>PSAAIYNIDTSSESPDHYLVDHTLDGRVLFPATGYLSIVWKTLARALGLGVEQLPVVFEDVVLHQATILPKTGTVSLEVRLLEASRAFEVSENGNLVVSGKVYQWDDPDPRLFDHPESPTPNPTEPLFLAQAEVYKELRLRGYDYGPHFQGILEASLEGDSGRLLWKDNWVSFMDTMLQMSILGSAKHGLYLPTRVTAIHIDPATHRQKLYTLQDKAQVADVVVSRWLRVTVAGGVHISGLHTESAPRRQQEQQVPILEKFCFTPHTEEGCLSERAALQEELQLCKGLVQALQTKVTQQGLKMVVPGLDGAQIPRDPSQQELPRLLSAACRLQLNGNLQLELAQVLAQERPKLPEDPLLSGLLDSPALKACLDTAVENMPSLKMKVVEVLAGHGHLYSRIPGLLSPHPLLQLSYTATDRHPQALEAAQAELQQHDVAQGQWDPADPAPSALGSADLLVCNCAVAALGDPASALSNMVAALREGGFLLLHTLLRGHPLGDIVAFLTSTEPQYGQGILSQDAWESLFSRVSLRLVGLKKSFYGSTLFLCRRPTPQDSPIFLPVDDTSFRWVESLKGILADEDSSRPVWLKAINCATSGVVGLVNCLRREPGGNRLRCVLLSNLSSTSHVPEVDPGSAELQKVLQGDLVMNVYRDGAWGAFRHFLLEEDKPEEPTAHAFVSTLTRGDLSSIRWVCSSLRHAQPTCPGAQLCTVYYASLNFRDIMLATGKLSPDAIPGKWTSQDSLLGMEFSGRDASGKRVMGLVPAKGLATSVLLSPDFLWDVPSNWTLEEAASVPVVYSTAYYALVVRGRVRPGETLLIHSGSGGVGQAAIAIALSLGCRVFTTVGSAEKRAYLQARFPQLDSTSFANSRDTSFEQHVLWHTGGKGVDLVLNSLAEEKLQASVRCLATHGRFLEIGKFDLSQNHPLGMAIFLKNVTFHGVLLDAFFNESSADWREVWALVQAGIRDGVVRPLKCTVFHGAQVEDAFRYMAQGKHIGKVVVQVLAEEPEAVLKGAKPKLMSAISKTFCPAHKSYIIAGGLGGFGLELAQWLIQRGVQKLVLTSRSGIRTGYQAKQVRRWRRQGVQVQVSTSNISSLEGARGLIAEAAQLGPVGGVFNLAVVLRDGLLENQTPEFFQDVCKPKYSGTLNLDRVTREACPELDYFVVFSSVSCGRGNAGQSNYGFANSAMERICEKRRHEGLPGLAVQWGAIGDVGILVETMSTNDTIVSGTLPQRMASCLEVLDLFLNQPHMVLSSFVLAEKAAAYRDRDSQRDLVEAVAHILGIRDLAAVNLDSSLADLGLDSLMSVEVRQTLERELNLVLSVREVRQLTLRKLQELSSKADEASELACPTPKEDGLAQQQTQLNLRSLLVNPEGPTLMRLNSVQSSERPLFLVHPIEGSTTVFHSLASRLSIPTYGLQCTRAAPLDSIH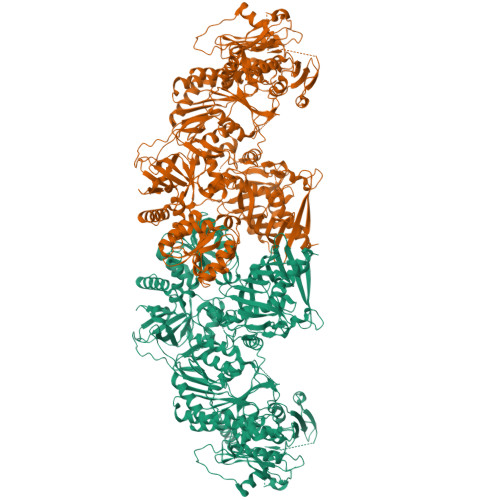SLAAYYIDCIRQVQPEGPYRVAGYSYGACVAFEMCSQLQAQQSPAPTHNSLFLFDGSPTYVLAYTQSYRAKLTPGCEAEAETEAICFFVQQFTDMEHNRVLEALLPLKGLEERVAAAVDLIIKSHQGLDRQELSFAARSFYYKLRAAEQYTPKAKYHGNVMLLRAKTGGAYGEDLGADYNLSQVCDGKVSVHVIEGDHRTLLEGSGLESIISIIHSSLAEPRVSVREG[2x]>SHMALRVGIVYGTRPEAIKLAPLVLALDADPGFEPVIITTGQHRDMLDEINELFGLRPRHNLDIMRPGQRLSAMASRIVGELGDPLLDELVDVAVVQGDTSTAFAAAYAAACERIPVAHLEAGLRTGDRFEPFPEEINRRLITQLADLHFAPTADAAGNLLAEGVRSDDVYVTGNTVIDAMHLVLDRPGDSANRELDAFTEGRQTVLLTMHRRESWGIPMGRVAAAVAELCRSRPTLRFVIPLHPNPEVRRVFRSHLSSLTQVLLCEPLRYSEFIRLMHRAVLVLTDSGGVQEEAPTLGKPVLVLRDRTERPEGIAAGCARLVGTDPALIVKEVGRLLDDPEAYEAMRRPGIVCYGEGDAAARCLEALRER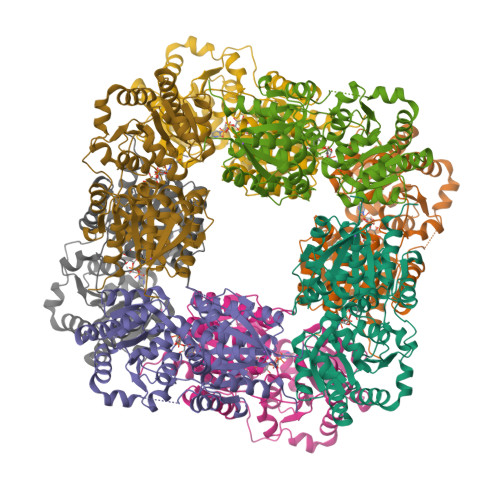WLSSPDASAGLRTYR[8x]>MAYVEIIEQPKQRGMRFRYKCEGRSAGSIPGERSTDTTKTHPTIKINGYTGPGTVRISLVTKDPPHRPHPHELVGKDCRDGYYEADLCPDRSIHSFQNLGIQCVKKRDLEQAISQRIQTNNNPFHVPIEEQRGDYDLNAVRLCFQVTVRDPAGRPLLLTPVLSHPIFDNRAPNTAELKICRVNRNSGSCLGGDEIFLLCDKVQKEDIEVYFTGPGWEARGSFSQADVHRQVAIVFRTPPYADPSLQAPVRVSMQLRRPSDRELSEPMEFQYLPD[2x];>MGPYLQILEQPKQRGFRFRYVCEGPSHGGLPGASSEKNKKSYPQVKICNYVGPAKVIVQLVTNGKNIHLHAHSLVGKHCEDGVCTVTAGPKDMVVGFANLGILHVTKKKVFETLEARMTEACIRGYNPGLLVHSDLAYLQAEGGGDRQLTDREKEIIRQAAVQQTKEMDLSVVRLMFTAFLPDSTGSFTRRLEPVVSDAIYDSKAPNASNLKIVRMDRTAGCVTGGEEIYLLCDKVQKDDIQIRFYEEEENGGVWE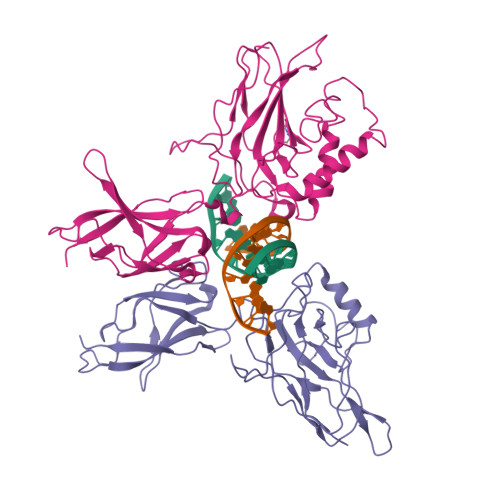GFGDFSPTDVHRQFAIVFKTPKYKDVNITKPASVFVQLRRKSDLETSEPKPFLYYPE[2x]> FYKREMFDPAEEYKMNHKRRGLALIFNQKRFD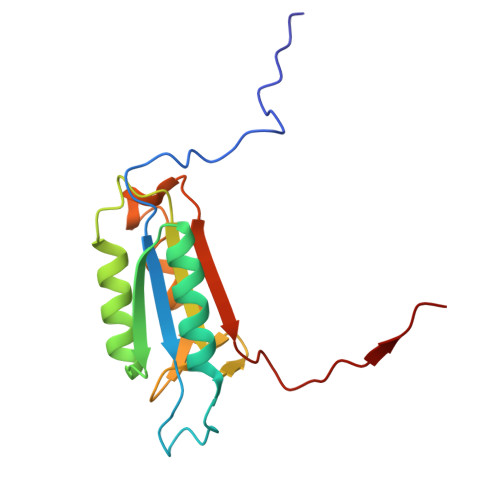WKLGLKTRNGTDKDRDNLERRFQELGFEVKAYNDLSAEEVLEKIQEASTADHSDADCFVCVFLSHGEDGHVYANDAKIEIQELTNLFKGDKCQSLVGKPKIFIIQACRGDKLDDAVTPM>[2x]SGISLDNSYKMDYPEMGLCIIINNKNFHKSTGMTSRSGTDVDAANLRETFRNLKYEVRNKNDLTREEIVELMRDVSKEDHSKRSSFVCVLLSHGEEGIIFGTNGPVDLKKITNFFRGDRCRSLTGKPKLFIIQACRGTELDCGIE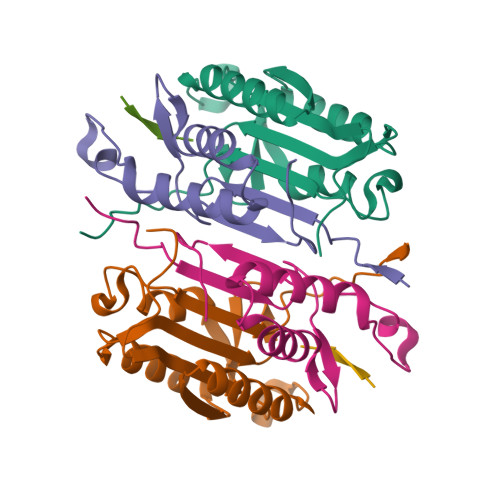TD;>[2x]SGVDDDMACHKIPVEADFLYAYSTAPGYYSWRNSKDGSWFIQSLCAMLKQYADKLEFMHILTRVNRKVATEFESFSFDATFHAKKQIPCIVSMLTKELYFYH;>XITVKD[2x]> HSQG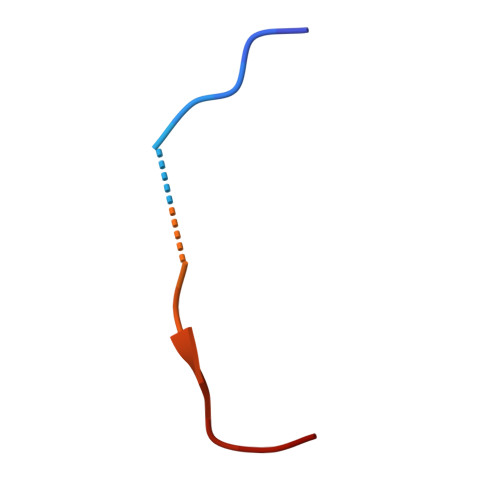TFTSDYSKYLDSRRAQDFVQWLMNT>[2x]ADSTSGWRAPSCTKVTGDGAVTFTTDDGATLAPTTGTLQSVSYTHGLVALDTPNTLLATHNDELQRSTDAGCTWTKVAT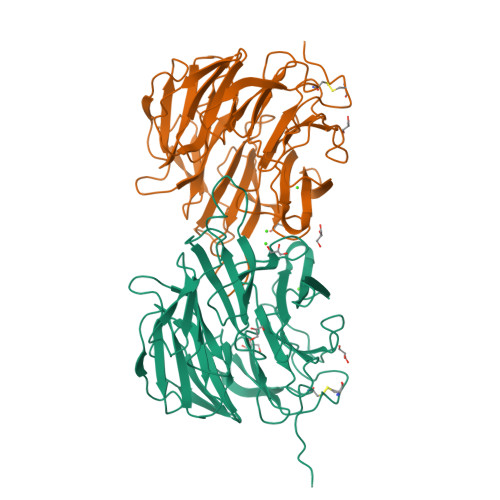LGSGSTWLTAATGGRAFAWEKNGGYLARVDGRTVTKLSSPSADIVGVGTDKARRDHVRLAGSDGQLYDSTDAGATWKPLGKLAFGPGASVYTVSFDPADLDHAVAGGMTTGGAVTTDGGATWTAATGLSATAGGKSNLFAASVSPADRNVVYALGIDLVEAAPNSGAEGRHLYRSTDGGRTYTRIVDDTPDTELTNSTLLAPSPVDPNVLYFEYGTYFQAYGTDLYRYDARTGKVGKTHNAHDGISAIAFNPARPSVMYLGLEEVQIHH> SESKVKKVVSIPAIDEG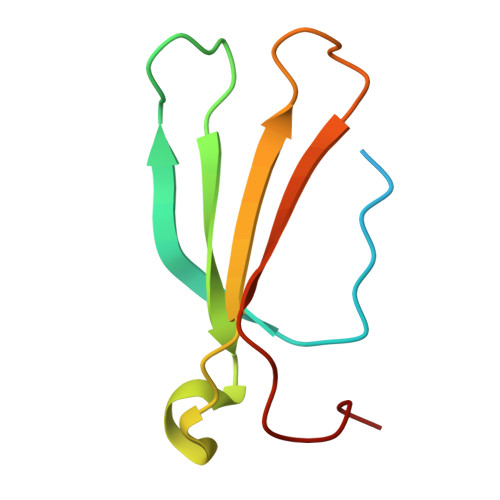DLWTWRKYGQKDILGSRFPRGYYRCAYKFTHGCKATKQVQRSETDSNMLAITYLSEHNHPRPT>MKFTVEREHLLKPLQQVSGPLGGRPTLPILGNLLLQVADGTLSLTGTDLEMEMVARVALVQPHEPGATTVPARKFFDICRGLPEGAEIAVQLEGERMLVRSGRSRFSLSTLPAADFPNLDDWQSEVEFTLPQATMKRLIEATQFSMAHQDVRYYLNGMLFETEGEELRTVATDGHRLAVCSMPIGQSLPSHSVIVPRKGVIELMRMLDGGDNPLRVQIGSNNIRAHVGDFIFTSKLVDGRFPDYRRVLPKNPDKHLEAGCDLLKQAFARAAILSNEKFRGVRLYVSENQLKITANNPEQEEAEEILDVTYSGAEME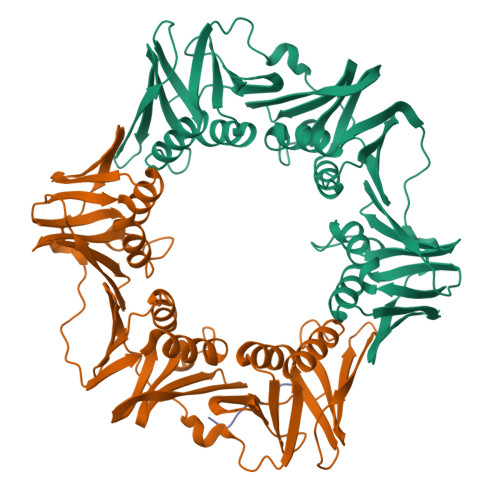IGFNVSYVLDVLNALKCENVRMMLTDSVSSVQIEDAASQSAAYVVMPMRL[2x];> VTLLDPQMERQLVLGL> MGCQSTQLQTPAPDTGGIVELNRQLGRGVNLGNALEAPWEGAWGVRLEEGFFELIREAGFKTIRLPVSWTHHAGRAAPYTIDPAFFSRVDWAVTQATRRGLNIVVNVHHYDELNANPQAEEARYLSIWRQIAERYRNQPGSVYFELLNEPHGRFNDNPQLWNDLLAKALRVVRESNPSRAVIVGPVGWNSLWRLSELRLPDDPNLIVTFHYYDPLEFTHQGAEWLNPVPPTGVVWRENQGAFAAGWQNWSWGSRVGFVGEALEITYQEGWAGFYLHSDAGVEGYDRLAFRTSAPVSLQVSCRRDAPAKAVTTSGGVETVVNLSECGNPSRLTDLILQN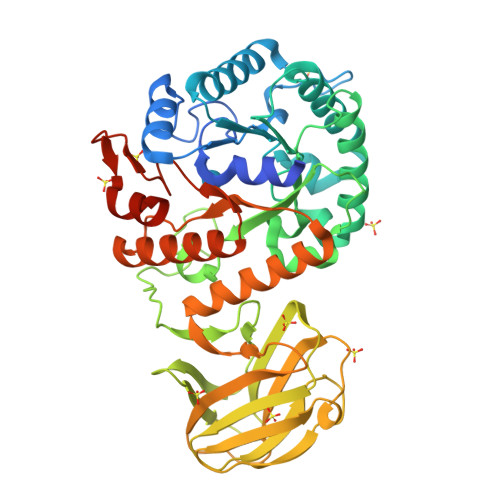NSPNARAAFRLERLELRGPGSPLALLTHQQNAIAQAMEFAQRWAEQNRRPIFVGEFGAYEKGDLDSRVRWTGAVRSELEKRNFSWAYWEFAAGFGIYDRTTRQWRTPLLKALVPEQPKLAAALEHHHHHH RfaH, a paralog of the universally conserved NusG, binds to RNA polymerases (RNAP) and ribosomes to activate expression of virulence genes. In free, autoinhibited RfaH, an α-helical KOW domain sequesters the RNAP-binding site. Upon recruitment to RNAP paused at an ops site, KOW is released and refolds into a β-barrel, which binds the ribosome. RfaH recruitment requires a 12-nucleotide (nt) operon polarity suppressor (ops) sequence, which induces RNAP pausing.

We wondered how strongly the initial docking of RfaHCC onto the opsHP drives upstream DNA melting and hybrid expansion. Therefore, we assembled an EC on a scaffold in which a WC bp in the upstream DNA would have to be disrupted and formation of a non-WC C:U pair would have to be “forced” into the 11-bp hybrid. Strikingly, the 3.1 Å structure revealed that the ensuing RfaHCC-bound complex was virtually identical to opsPECEnc, with the 11-bp hybrid, even though the C:U bp does not energetically fully compensate for the lost DNA bp. We conclude that docking of RfaH provides a strong driving force for hybrid expansion, leading to a hyper-paused opsPECEnc.

>[2x]MQGSVTEFLKPRLVDIEQVSSTHAKVTLEPLERGFGHTLGNALRRILLSSMPGCAVTEVEIDGVLHEYSTKEGVQEDILEILLNLKGLAVRVQGKDEVILTLNKSGIGPVTAADITHDGDVEIVKPQHVICHLTDENASISMRIKVQRGRGYVPASTRIHSEEDERPIGRLLVDACYSPVERIAYNVEAARVEQRTDLDKLVIEMETNGTIDPEEAIRRAATILAEQLEAFVDLRDVRQPEVKEEKPEFDPILLRPVDDLELTVRSANCLKAEAIHYIGDLVQRTEVELLKTPNLGKKSLTEIKDVLASRGLSLGMRLENWPPASIADE;> MVYSYTEKKRIRKDFGKRPQVLDVPYLLSIQLDSFQKFIEQDPEGQYGLEAAFRSVFPIQSYSGNSELQYVSYRLGEPVFDVQECQIRGVTYSAPLRVKLRLVIYEREAPEGTVKDIKEQEVYMGEIPLMTDNGTFVINGTERVIVSQLHRSPGVFFDSDKGKTHSSGKVLYNARIIPYRGSWLDFEFDPKDNLFVRIDRRRKLPATIILRALNYTTEQILDLFFEKVIFEIRDNKLQMELVPERLRGETASFDIEANGKVYVEKGRRITARHIRQLEKDDVKLIEVPVEYIAGKVVAKDYIDESTGELICAANMELSLDLLAKLSQSGHKRIETLFTNDLDHGPYISETLRVDPTNDRLSALVEIYRMMRPGEPPTREAAESLFENLFFSEDRYDLSAVGRMKFNRSLLREEIEGSGILSKDDIIDVMKKLIDIRNGKGEVDDIDHLGNRRIRSVGEMAENQFRVGLVRVERAVKERLSLGDLDTLMPQDMINAKPISAAVKEFFGSSQLSQFMDQNNPLSEITHKRRISALGPGGLTRERAGFEVRDVHPTHYGRVCPIETPEGPNIGLINSLSVYAQTNEYGFLETPYRKVTDGVVTDEIHYLSAIEEGNYVIAQANSNLDEEGHFVEDLVTCRSKGESSLFSRDQVDYMDVSTQQVVSVGASLIPFLEHDDANRALMGANMQRQAVPTLRADKPLVGTGMERAVAVDSGVTAVAKRGGVVQYVDASRIVIKVNEDEMYPGEAGIDIYNLTKYTRSNQNTCINQMPCVSLGEPVERGDVLADGPSTDLGELALGQNMRVAFMPWNGYNFEDSILVSERVVQEDRFTTIHIQELACVSRDTKLGPEEITADIPNVGEAALSKLDESGIVYIGAEVTGGDILVGKVTPKGETQLTPEEKLLRAIFGEKASDVKDSSLRVPNGVSGTVIDVQVFTRDGVEKDKRALEIEEMQLKQAKKDLSEELQILEAGLFSRIRAVLVAGGVEAEKLDKLPRDRWLELGLTDEEKQNQLEQLAEQYDELKHEFEKKLEAKRRKITQGDDLAPGVLKIVKVYLAVKRRIQPGDKMAGRHGNKGVISKINPIEDMPYDENGTPVDIVLNPLGVPSRMNIGQILETHLGMAAKGIGDKINAMLKQQQEVAKLREFIQRAYDLGADVRQKVDLSTFSDEEVMRLAENLRKGMPIATPVFDGAKEAEIKELLKLGDLPTSGQIRLYDGRTGEQFERPVTVGYMYMLKLNHLVDDKMHARSTGSYSLVTQQPLGGKAQFGGQRFGEMEVWALEAYGAAYTLQEMLTVKSDDVNGRTKMYKNIVDGNHQMEPGMPESFNVLLKEIRSLGINIELEDE;> VKDLLKFLKAQTKTEEFDAIKIALASPDMIRSWSFGEVKKPETINYRTFKPERDGLFCARIFGPVKDYECLCGKYKRLKHRGVICEKCGVEVTQTKVRRERMGHIELASPTAHIWFLKSLPSRIGLLLDMPLRDIERVLYFESYVVIEGGMTNLERQQILTEEQYLDALEEFGDEFDAKMGAEAIQALLKSMDLEQECEQLREELNETNSETKRKKLTKRIKLLEAFVQSGNKPEWMILTVLPVLPPDLRPLVPLDGGRFATSDLNDLYRRVINRNNRLKRLLDLAAPDIIVRNEKRMLQEAVDALLDNGRRGRAITGSNKRPLKSLADMIKGKQGRFRQNLLGKRVDYSGRSVITVGPYLRLHQCGLPKKMALELFKPFIYGKLELRGLATTIKAAKKMVEREEAVVWDILDEVIREHPVLLNRAPTLHRLGIQAFEPVLIEGKAIQLHPLVCAAYNADFDGDQMAVHVPLTLEAQLEARALMMSTNNILSPANGEPIIVPSQDVVLGLYYMTRDCVNAKGEGMVLTGPKEAERLYRSGLASLHARVKVRITEYEKDANGELVAKTSLKDTTVGRAILWMIVPKGLPYSIVNQALGKKAISKMLNTCYRILGLKPTVIFADQIMYTGFAYAARSGASVGIDDMVIPEKKHEIISEAEAEVAEIQEQFQSGLVTAGERYNKVIDIWAAANDRVSKAMMDNLQTETVINRDGQEEKQVSFNSIYMMADSGARGSAAQIRQLAGMRGLMAKPDGSIIETPITANFREGLNVLQYFISTHGARKGLADTALKTANSGYLTRRLVDVAQDLVVTEDDCGTHEGIMMTPVIEGGDVKEPLRDRVLGRVTAEDVLKPGTADILVPRNTLLHEQWCDLLEENSVDAVKVRSVVSCDTDFGVCAHCYGRDLARGHIINKGEAIGVIAAQSIGEPGTQLTMRTFHIGGAASRAAAESSIQVKNKGSIKLSNVKSVVNSSGKLVITSRNTELKLIDEFGRTKESYKVPYGAVLAKGDGEQVAGGETVANWDPHTMPVITEVSGFVRFTDMIDGQTITRQTDELTGLSSLVVLDSAERTAGGKDLRPALKIVDAQGNDVLIPGTDMPAQYFLPGKAIVQLEDGVQISSGDTLARIPQESGGTKDITGGLPRVADLFEARRPKEPAILAEISGIVSFGKETKGKRRLVITPVDGSDPYEEMIPKWRQLNVFEGERVERGDVISDGPEAPHDILRLRGVHAVTRYIVNEVQDVYRLQGVKINDKHIEVIVRQMLRKATIVNAGSSDFLEGEQVEYSRVKIANRELEANGKVGATYSRDLLGITKASLATESFISAASFQETTRVLTEAAVAGKRDELRGLKENVIVGRLIPAGTGYAYHQDRMRRRAAGEAPAAPQVTAEDASASLAELLNAGLGGSDNELEVHHHHHH;> MARVTVQDAVEKIGNRFDLVLVAARRARQMQVGGKDPLVPEENDKTTVIALREIEEGLINNQILDVRERQEQQEQEAAELQAVTAIAEGRR;> GHMQSWYLLYCKRGQLQRAQEHLERQAVNCLAPMITLEKIVRGKRTAVSEPLCPNYLFVEFDPEVIHTTTINATRGVSHFVRFGASPAIVPSAVIHQLSVYKPKDIVDPATPYPGDKVIITEGAFEGFQAIFTEPDGEARCMLLLNLINKEIKHSVKNTEFRKL> SNAPDSLMKVSIPDFEKEGEGKSKHVMYKIKVKTGGEEWAVYRRYSDFYWLHKKLQQRYPELVPELPPKKWI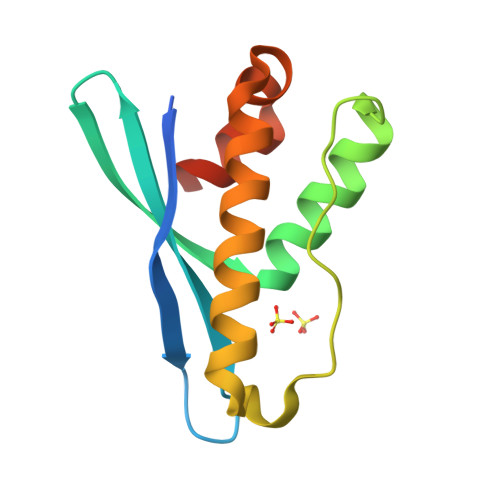YSALDEQILEKRKQGLEKYIQRIVSHPVLANDELVVSFLQAKAEHTG> GPHMTRKLFVGGNWKMNGSYSHINTFFDTLQKADTDPNADIVIGVPACYLKYAQDKAPKGIKIAAENCYKVGSGAFTGEISTEMIKDCGCEWVILGHSERRHIFGESNELIGEKVKHALDSGLNVIPCIGELLSEREAG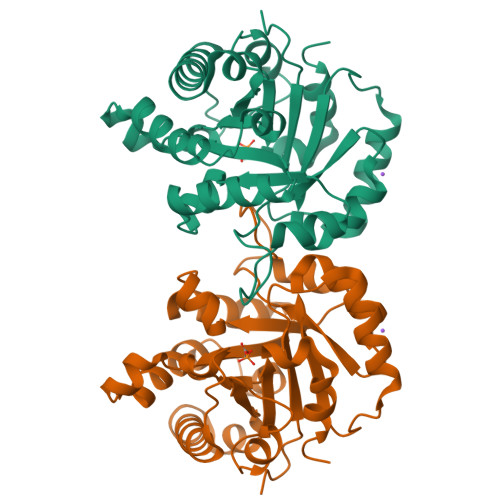KTNDVCFAQMDAIAKNVPSKEAWDKVVIAYEPVWAIGTGKTATPAQAQEVHKVVRDWIRKHVDAGIADKVRILYGGSVTASNAKDLGTQPDVDGFLVGGASLKPDFITIINARR> MSWELVATVLGSVSVLVGAVVFLGGAIGLLRFPDLYVRSSAIGAAAGLGLVFVIA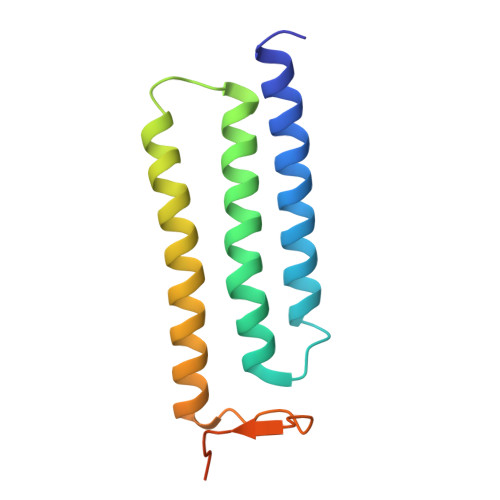GAFLLHPTWEAAPKVAVAAILQFASSAIGAMYIARAGFLSGAAPTTATRYSQIEFTTGPPTDSTEVTRDD>[4x]GSFVGSIDQGTTSSRFLIFNGEGNPVASHQIEFENLYPKSGWHEQDPYELLNSVQQCIDGAMHKFASLGYSKENIRAIGITNQRETTVVWDSVTGEPLHNAIVWPDTRTSALVRELKARQSADSLLELCGLPLSTYPSSVKLLWLIQNVDAVKQAYEEGRLAFGTVDSWLIYKLNGGAQAERPIHVTDSTNASRTMFMNLRTLQYDDKLLGFFGIDRNKIKLPKIVPSSDPEAFGKVATGALAGVPIAGCLGDQSSALVGQCGFSPGQAKNTYGTGCFLLYNVGTEPVISKYGLLAT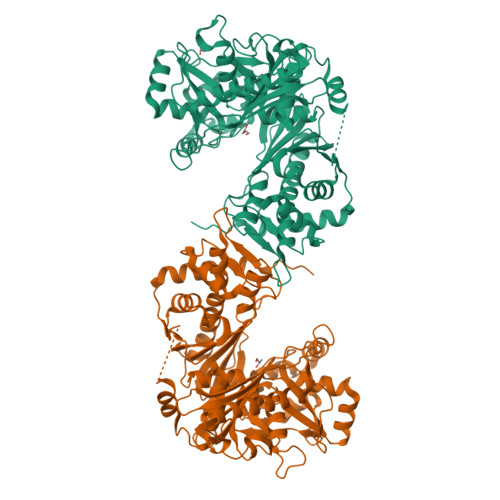VAYDFGRGRKPVYALEGSIAVAGAGITFLMNNLGFAPKPSEINALAESVLDNGGVVFVTAFSGLFAPYWIDDAKGTLFGITQHTTKGHIARATLEATCYQTRAILDAMEKDSGHKLESLAVDGGLSASDLCMQTQADISGIPVDRPRMRETTALGAAIAAGLATGVWRELDHVKESIAGGANGNGKKNAREVFYPKMDRKKAERLFRKWEQAVEMSRGWVREQEEEDGE>[2x]MKHHHHHHSAGLEVLFQGPGTGSEFMMFGKKKNNGGSSTARYSAGNKYNTLSNNYALSAQQLLNASKIDDIDSMMGFERYVPPQYNGRFDAKDIDQIPGRVGWLTNMHATLVSQETLSSGSNGGGNSNDGERVTTNQGISGVDFYFLDEEGGSFKSTVVYDPYFFIACNDESRVNDVEELVKKYLESCLKSLQIIRKEDLTMDNHLLGLQKTLIKLSFVNSNQLFEARKLLRPILQDNANNNVQRNIYNVAANGSEKVDAKHLIEDIREYDVPYHVRVSIDKDIRVGKWYKVTQQGFIEDTRKIAFADPVVMAFAIATTKPPLKFPDSAVDQIMMISYMIDGEGFLITNREIISEDIEDFEYTPKPEYPGFFTIFNENDEVALLQRFFEHIRDVRPTVISTFNGDFFDWPFIHNRSKIHGLDMFDEIGFAPDAEGEYKSSYCSHMDCFRWVKRDSYLPQGSQGLKAVTQSKLGYNPIELDPELMTPYAFEKPQHLSEYSVSDAVATYYLYMKYVHPFIFSLCTIIPLNPDETLRKGTGTLCEMLLMVQA;>MSINLHSAPEYDPSYKLIQLTPELLDIIQDPVQNHQLRFKSLDKDKSEVVLCSHDKTWVLKQRKHSNTVLLMREFVPEQPITFDETL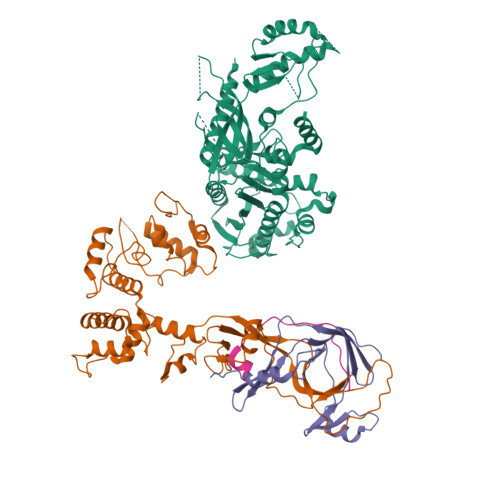LFGLSKPYMDVVGFAKTESEFETRETHGELNLNSVPIYNGELDFSDKIMKRSSTKVIGTLEELLENSPCSALEGISKWHKIGGSVKDGVLCILSQDFLFKALHVLLMSAMAESLDLQHLNVEDTHHAVGKDIEDEFNPYTREIIETVLNKFAVQEQEAENNTWRLRIPFIAQWYGIQALRKYVSGISMPIDEFLIKWKSLFPPFFPCDIDIDMLRGYHFKPTDKTVQYIAKSTLPMDPKERFKVLFRLQSQWDLEDIKPLIEELNSRGMKIDSFIMKYARRKRLGKKTVVTSR[2x];>MPSVDIDASQWQKLTQSREKQTTVITPLGMMMLEIQGELELPKDFASLARRDSPNEGRFSEQDGETLIRFGSLQIDGERATLFVGKKQRLLGKVTKLDVPMGIMHFNSKDNKVELVDVMKYKVIFKDRPLPIM[2x];>[2x]GAMGNQTVKIWVKYNEGFSNAVRKNVTWNNLWE> PKVSVIMTSYNKSDYVAKSISSILSQTFSDFELFIMDDNSNEETLNVIRPFLNDNRVRFYQSDISGVKERTEKTRYAALINQAIEMAEGEYITYATDDNIYMPDRLLKMVRELDTHPEKAVIYSASKTYHLNENRDIVKETVRPAAQVTWNAPCAIDHCSVMHRYSVLEKVKEKFGSYWDESPAFYRIGDARFFWRVNHFYPFYPLDEELDLNYITDQSIHFQLFELEKNEFVRNLP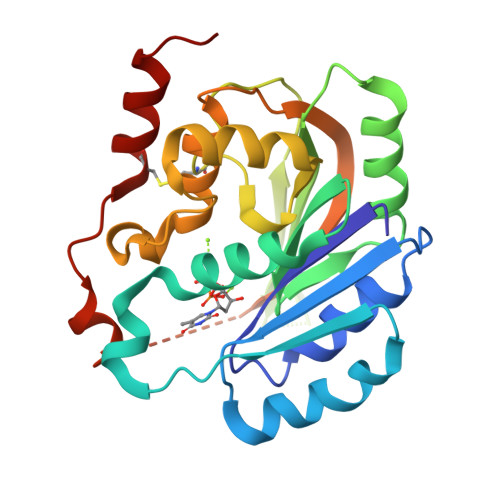PQRNCRELRESLKKLGMG>[5x]GSHMEEKRLSAKKGLPPGTLVYTGKYREDFEIEVMNY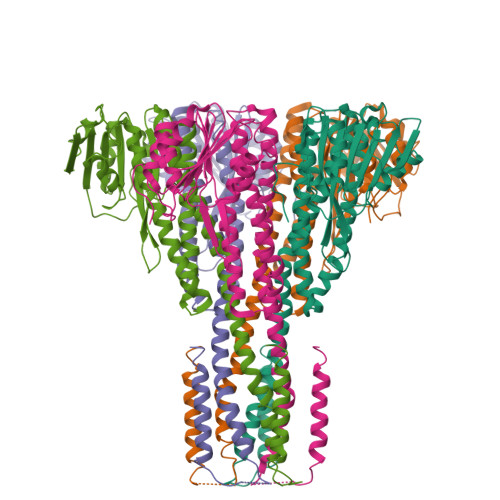SIEEFREFKTTDVESVLPFRDSSTPTWINITGIHRTDVVQRVGEFFGIHPLVLEDILNVHQRPKVEFFENYVFIVLKMFTYDKNLHELESEQVSLILTKNCVLMFQEKIGDVFDPVRERIRYNRGIIRKKRADYLLYSLIDALVDDYFVLLEKIDDEIDVLEEEVLERPEKETVQRTHQLKRNLVELRKTIWPLREVLSSLYRDVPPLIEKETVPYFRDVYDHTIQIADTVETFRDIVSGLLDVYLSSVSNKTNEVMKVLTIIATIFMPLTFIAGIYGMNFEYMPELRWKWGYPVVLAVMGVIAVIMVVYFKKKKWL>MPPRPLDVLNRSLKSPVIVRLKGGREFRGTLDGYDIHMNLVLLDAEEIQNGEVVRKVGSVVIRGDTVVF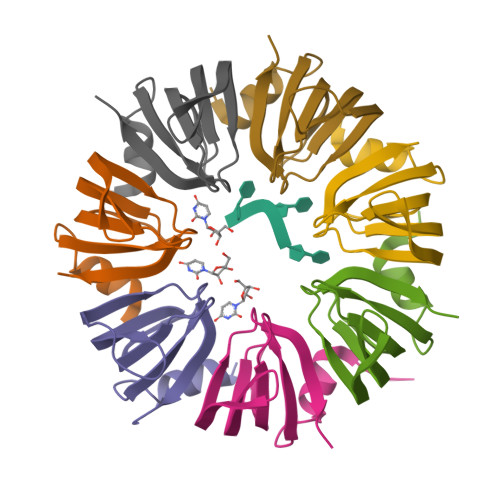VSPAPGGE[14x]[(5Z)-5-{[3-(carboxymethoxy)-4-methoxyphenyl]methylidene}-2,4-dioxo-1,3-thiazolidin-3-yl]acetic acid | C15 H13 N O8 S 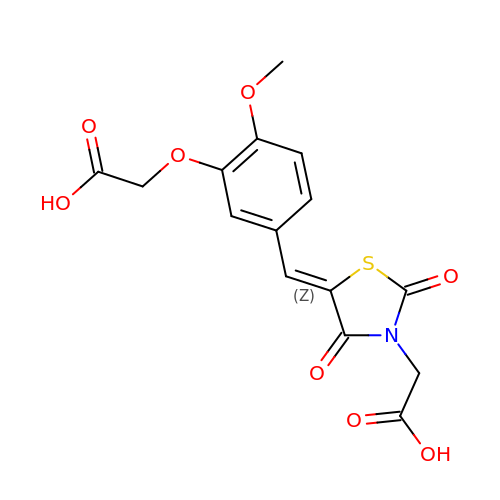| DLKPSHJFPIKYCB-WZUFQYTHSA-N>MSFPGWGPYPPVERDETSAITYSSKLHGSVTVRDPYSQLEVPFEDSEETKAFVHSQRKFARTYLDENPDREAWLETLKKSWNYRRFSALKPESDGHYYFEYNDGLQSQLSLYRVRMGEEDTVLTESGPGGELFFNPNLLSLDGNAALTGFVMSPCGNYWAYGVSEHGSDWMSIYVRKTSSPHLPSQERGKDPGRMNDKIRHVRFFIVSWTSDSKGFFYSRYPPEDDEGKGNAPAMNCMVYYHRIGEDQESDVLVHEDPEHPFWISSVQLTPSGRYILFAASRDASHTQLVKIADLHENDIGTNMKWKNLHDPWEARFTIVGDEGSKIYFMTNLKAKNYKVATFDANHPDEGLTTLIAEDPNAFLVSASIHAQDKLLLVYLRNASHEIHIRDLTTGKPLGRIFEDLLGQFMVSGRRQDNDIFVLFSSFLSPGTVYRYTFGEEKGYRSLFRAISIPGLNLDDFMTESVFYPSKDGTSVHMFITRPKDVLLDGTSPVLQYGYGGFSLAMLPTFSLSTLLFCKIYRAIYAIPNIRGGSEYGESWHREGMLDKKQNVFDDFNAATEWLIANKYASKDRIAIRGGANGGVLTTACANQAPGLYRCVITIEGIIDMLRFPKFTFGASWRSEYGDPEDPEDFDFIFKYSPYHNIPPPGDTVMPAMLFFTAAYDDRVSPLHTFKHVAALQHNFPKGPNPCLMRIDLNSGHFAGKSTQEMLEETADEYSFIGKSMGLTMQTQGSVDSSRWSCVTV[4x];>WVIVVGVIGVIGSVMSTE[4x]

OphP is an essential enzyme for the biosynthesis of the macrocyclic peptide natural product omphalotin A. The enzyme has been proposed to proteolytically release a peptide intermediate from the precursor protein OphMA and to macrocyclize the multiply α-N-methylated core of this intermediate to produce omphalotin A. Our *in vitro* experiments demonstrate that OphP does not process OphMA but shows robust macrocyclase activity on pre-processed α-N-methylated peptides. OphP tolerates sequence promiscuity in the substrate but has a preference for highly α-N-methylated substrates and for N-methylated glycine residue at the catalytic site. The promiscuity of OphP is explained by structural analysis of co-complexes which reveals a predominantly hydrophobic substrate binding cleft with few interactions between substrate side chains and OphP. Similar to other POPs, the monomer has two domains, an α/β hydrolase domain (residues 1–82, 453–738) and the seven-bladed β-propeller domain (residues 83–452) ([Fig fig4]).

To characterize the interactions of OphP with its presumed natural substrate, S580A mutant crystals were soaked with a ten-fold methylated Oph-18mer^NL^ (W1-^me^V2-I3-^me^V4-^me^V5-^me^G6-^me^V7-^me^I8-^me^G9-V10-^me^I11-^me^G12-S13-^me^V14-M15-S16-T17-E18) and a seven-fold methylated Oph-15mer substrate (G1-F2-P3-W4-^me^V5-I6-^me^V7-^me^V8-^me^G9-^me^V10-^me^I11-^me^G12-V13-I14-G15) ([Fig fig2]) (both substrates yield dodecameric macrocycles with the underlined residues). The Oph-18mer^NL^ complex was obtained at 2.0 and the Oph-15mer complex at 2.5 Å resolution. The substrate peptide is located at the interface between two domains with its N-terminus extending into the β-propeller domain and its C-terminus contacting the hydrolase domain ([Fig fig4]). For Oph-18mer^NL^, we focus on subunit A which has the clearest density for the substrate ([Fig fig4]). Only residues ^me^I8-^me^G9-V10-^me^I11-^me^G12-S13-^me^V14 were fitted to the electron density whilst the remainder were presumed to be disordered ([Fig fig4]). The side chain of ^me^I8 packs against Arg316 whilst ^me^G9 makes almost no contact; the side chain of V10 interacts strongly with the aromatic ring of Phe617, ^me^I11 makes a similar interaction with Phe502 whilst its N-methyl group points to solvent ([Fig fig4]). The N-methyl group ^me^G12 contacts the indole ring of Trp621 and sits in the P1 pocket which is also formed by Ile606 and Phe502. The peptide bond of ^me^G12 is positioned for nucleophilic attack by Ser580. The hydroxyl of Tyr499 and the backbone amide of Asn581 are well-positioned to function as the canonical oxyanion hole pair to stabilize the tetrahedral intermediate formed by the nucleophilic attack of Ser580. ^me^Gly12 binds to a hydrophobic pocket formed by Trp621, Tyr625, Val668, Asn581, Phe502 and Ile606 ([Fig fig5]).>MHHHHHHAMGTLTPHKTISFGSLTIDPVNRQVMLGGENVALSTADFDMLWELATHAGQIMDRDALLKNLRGVTYDGMDRSVDVAISRLRKKLLDNATEPYRIKTVRNKGYLFA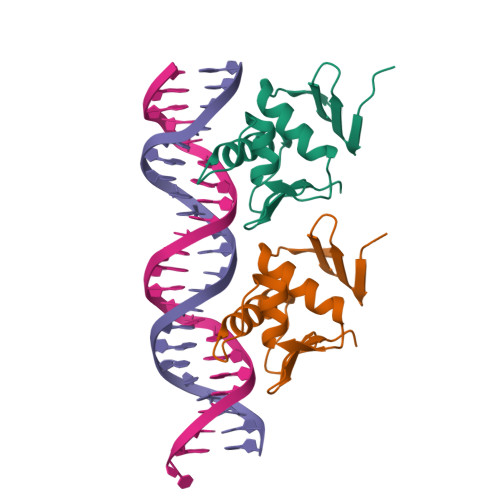PHAWDN[2x]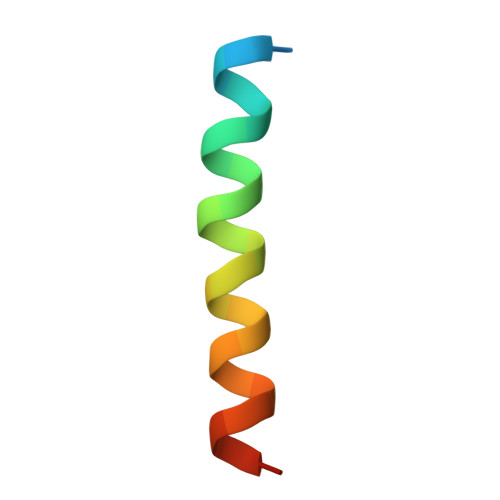> VPQDASTKKLSECLKRIGDELDSNMELQ>[8x]MDDLTIEILTDDADYDLQRFDCGEEALNLFLTTHLVRQHRNKILRAYILCRNTPERQVLGYYTLCGSCFERAALPSKSKQKKIPYKNIPSVTLGRLAIDRSLQGQGWDATLVAHAMNVVWSASLAVGIHGLFVEALNEKAHTFYKSLGFIPLVGENENALFFPTKSIELLFTQSDLEHHHHHH

AtaT is a type-II toxin from enterohemorrhagic E. coli, reported to acetylate the aminoacyl-moiety of initiator Met-tRNAfMet, thus inhibiting translation initiation. GNAT toxins acetylate the α-amino group of the aminoacyl-moiety of aminoacyl-tRNAs, using acetyl CoA (Ac-CoA) as the acetyl group donor, and inhibit cellular translation. The structural and biochemical studies revealed that the homodimerization of AtaT is required for both the enzymatic activity and the toxicity. Thus, AtaT has broader specificity toward aminoacyl-tRNAs, and the selection of substrate aminoacyl-tRNAs is governed by both the specific sequence in the acceptor stem and the side chain of the aminoacyl-moiety of aminoacyl-tRNAs.

To uncover the molecular basis of Met-tRNAfMet recognition by AtaT, AtaT, and acetyl–Met–tRNAfMet (Ac–Met–tRNAfMet) were co-crystallized and the structure was determined. Since Ac–Met–tRNAfMet is chemically more stable than Met–tRNAfMet, Ac–Met–tRNAfMet was used instead of Met–tRNAfMet for crystallization. The crystal belongs to the space group P21212 and contains eight AtaT molecules and two Ac–Met–tRNAfMet molecules in the asymmetric unit. The structure was model-built and refined to an R factor of 28.6% (Rfree = 34.1%) at 3.8 Å resolution. In the structure of AtaT complexed with Ac–Met–tRNAfMet, two tRNAfMet molecules (tRNAfMeta and tRNAfMetb) interact with an AtaT homodimer (AtaTa and AtaTb). The 3′-terminal single-stranded region and acceptor stem of each tRNAfMet interact with the positively charged interface between the two subunits of the AtaT dimer. In the complex structure, the α3 in AtaTb penetrates the major groove of the acceptor helix of tRNAfMeta, and the α1 in AtaTa also penetrates the groove from another angle. As a result, C1–A72 at the top of the acceptor helix of tRNAfMet are completely separated and the 5′-terminal C1 nucleoside is flipped. Residues S76, K77, S78, and K79 in α3 of AtaTb interact with the phosphate backbones of C67C68C69, at the bottom half of the acceptor helix. The 3′-C75A76–Ac–Met region of Ac–Met–tRNAfMet was disordered and not visible in the present structure.> VYRRKHQELQAMQMELQSPEYKLSKLRTSTIMTDYNPNYSFAGKTSSISDLKEVPRKNITLIRGLGHGAFGEVYEGQVSGMPNDPSPLQVAVKTLPEVCSEQDELDFLMEALIISKFNHQNIVRCIGVSLQSLPRFILLELMAGGDLKSFLRETRPRPSQPSSLAMLDLLHVARDIACGCQYLEENHFIHRDIAARNCLLTCPGPGRVAKIGDFGMARDIYRASYYRKG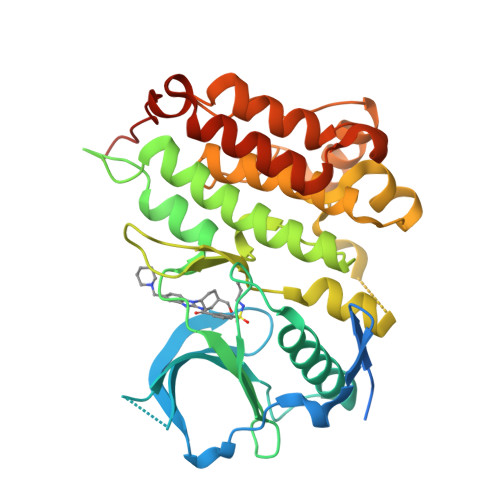GCAMLPVKWMPPEAFMEGIFTSKTDTWSFGVLLWEIFSLGYMPYPSKSNQEVLEFVTSGGRMDPPKNCPGPVYRIMTQCWQHQPEDRPNFAIILERIEYCTQDPDVINTALPIEYGPLVEEEEK>MPL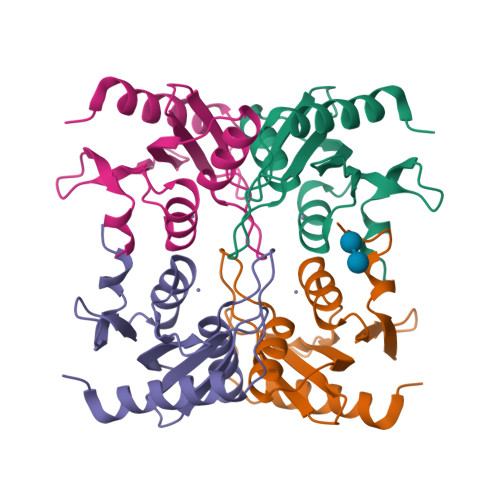SQEESTLIERATATINSIPISEDYSVASAALSSDGRIFTGVNVYHFTGGPCAELVVLGTAAAAAAGNLTCIVAIGNENRGILSPCGRCRQVLLDLHPGIKAIVKDSDGQPTAVGIRELLPSGYVWEG[4x]>[2x]MSPRSRLLASSLRGGLLLRPCSARRSTLLNPSPSPLRKAIFHTTSLRAFKNLAEIATSSKEDASSLKPKGKPSPPGDPLATIEKTAAEQRRADWAIIKQMSRYLWPKDSWSDKARVLLALSLLVGGKVLNVHVPFYFREIIDRLNIDVAAVGGTVSAVAGA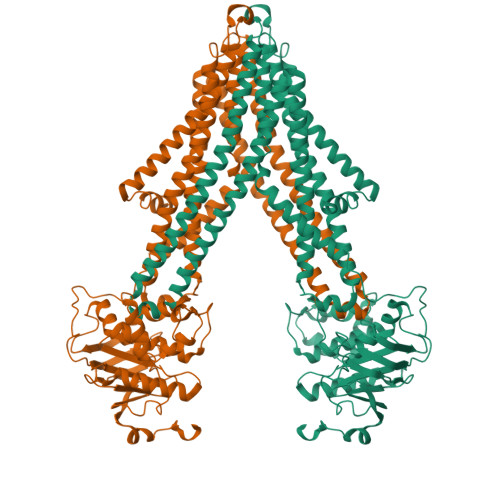VIFAYGASRIGAVVSQELRNAVFSSVAQKAIRRVATQTFGHLLNLDLSFHLSKQTGGLTRAIDRGTKGISYLLTSMVFHIVPTALEIGMVCGILTYQFGWEFAAITAATMAAYTAFTITTTAWRTKFRRQANAADNAASTVAVDSLINYEAVKYFNNEAYEIARYDKALQAYERSSIKVATSLAFLNSGQNIIFSSALTLMMWLGARGVLAGDLSVGDLVLINQLVFQLSVPLNFLGSVYRELRQSLLDMETLFDLQKVNVTIREAPNAKPLALPKGGEIRFENVTFGYYPDRPILRNLSLTIPAGKKVAVVGPSGCGKSTLLRLLFRSYDPQQGKIFIDDQDIKSVTLESLRKSIGVVPQDTPLFNDTVELNIRYGNVNATQEQVIAAAQKAHIHEKIISWPHGYQTRVGERGLMISGGEKQRLAVSRLILKDPPLLFFDEATSALDTHTEQALMANINEVVKEKKRTALFVAHRLRTIYDADLIIVLKEGVVVEQGSHRELMERDGVYAELWMAQEMLHQGEAAEEPAEGEKAEEKK> EVGKSFKDRKMIEKMQEENRKDREKAAAKFREYFPNFVGEP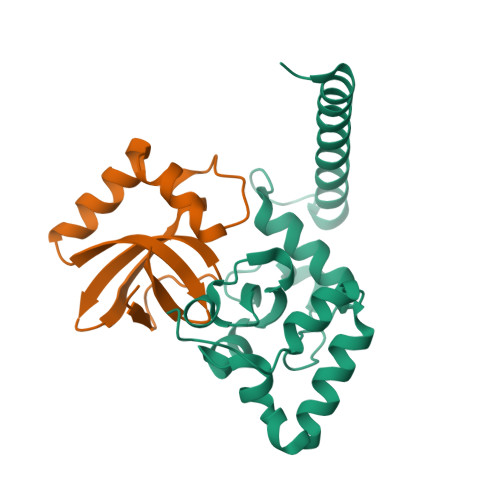KSKDILKLRLYEMQHGKCLYSGKEINLGRLNEKGYVEIDHALPFSRTWDDSFNNKVLVLGSENQNKGNQTPYEYFNGKDNSREWQEFKARVETSRFPRSKKQRILLQKFDEDGFKERNL;> MANKTYKIGKNAGYDGCGLCLAAISENEAIKVKYLRDICPDYDGDDKAEDWLRWGTDSRVKAAALEMEQYAYTSVGMASCWEFVEL(4R)-4-(4-cyanophenyl)-6-methyl-2-oxidanylidene-3-[2-oxidanylidene-2-(4-propan-2-ylpiperazin-1-yl)ethyl]-1-[3-(trifluoromethyl)phenyl]-4H-pyrimidine-5-carbonitrile | C29 H29 F3 N6 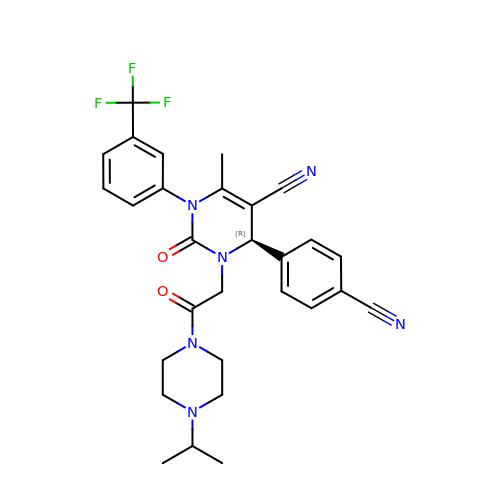O2 | MJSBQGLWAKMDDF-HHHXNRCGSA-N>NAQFLHTQVGRGLLGAVVNPLGEVTDKFAVTDNSEILYRPVDNAPPLYSERAAIEKPFLTGIKVIDSLLTCGEGQRMGIFASAGCGATFLMNMLIEHSGADIYVIGLIGERGREVTETVDYLKNSEKKSRCVLVYATSDYSSVDRCNAAYIATAIAEFFRTEGHKVALFIDSLTRYARALRDVALAAGESPARRGYPVSVFDSLPRLLERPGKLKAGGSITAFYTVLLEDDDFADPLAEEVRSILDGHIYLSRNLAQKGQFPAIDSLKSISRVFTQVVDEKHRIMAAAF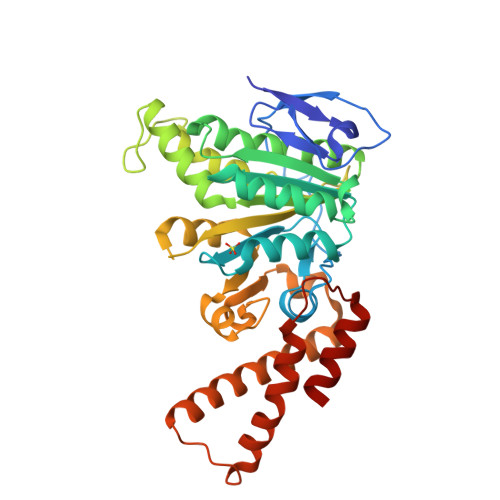RELLSEIEELRTIIDFGEYKPGENASQDKIYNKISVVESFLKQDYRLGFTYEQTMELIGETIR[2x]>RSPWEENFSRSYPCDEKKQNDSVIAECSNRRLQEVPQTVGKYVTELDLSDNFITHITNESFQGLQNLTKINLNHNPNVQHQNGNPGIQSNGLNITDGAFLNLKNLRELLLEDNQLPQIPSGLPESLTELSLIQNNIYNITKEGISRLINLKNLYLAWNCYFNKVCEKTNIEDGVFETLTNLELLSLSFNSLSHVPPKLPSSLRKLFLSNTQIKYISEEDFKGLINLTLLDLSGNCPRCFNAPFPCVPCDGGASINIDRFAFQNLTQLRYLNLSSTSLRKINAAWFKNMPHLKVLDLEFNYLVGEIASGAFLTMLPRLEILDLSFNYIKGSYPQHINISRNFSKLLSLRALHLRGYVFQELREDDFQPLMQLPNLSTINLGINFIKQIDFKLFQNFSNLEIIYLSENRISPLVKDTRQSYANSSSFQRHIRKRRSTDFEFDPHSNFYHFTRPLIKPQCAAYGKALDLSLNSIFFIGPNQFENLPDIACLNLSANSNAQVLSGTEFSAIPHVKYLDLT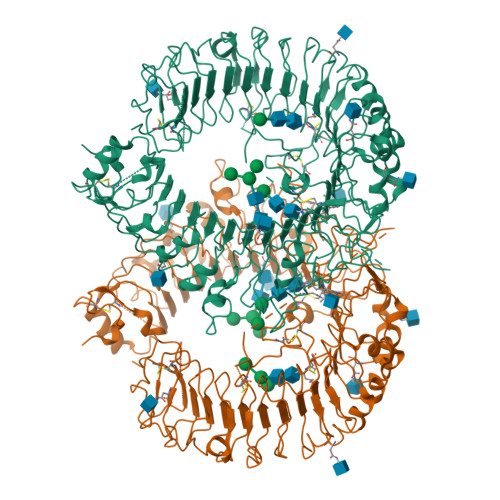NNRLDFDNASALTELSDLEVLDLSYNSHYFRIAGVTHHLEFIQNFTNLKVLNLSHNNIYTLTDKYNLESKSLVELVFSGNRLDILWNDDDNRYISIFKGLKNLTRLDLSLNRLKHIPNEAFLNLPASLTELHINDNMLKFFNWTLLQQFPRLELLDLRGNKLLFLTDSLSDFTSSLRTLLLSHNRISHLPSGFLSEVSSLKHLDLSSNLLKTINKSALETKTTTKLSMLELHGNPFECTCDIGDFRRWMDEHLNVKIPRLVDVICASPGDQRGKSIVSLELTTCVSDVTEFLVPR[2x]>[6x]GGUCACAACGGCUU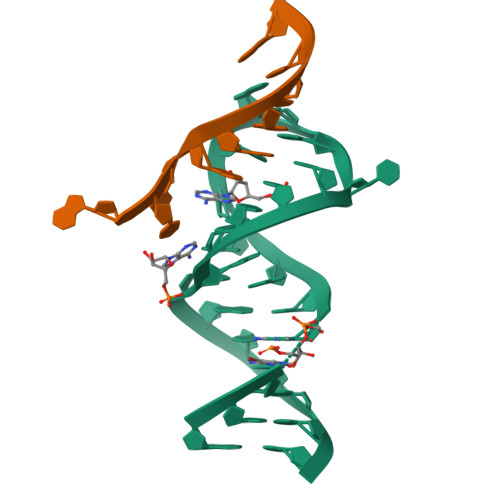CCUGGCGUGACC;>[6x]AUUGGAGCA> MRGLRKEALEELMKLLNMKDFPYRIEGIDISHLQGKYTVASLVVFEDGFPKKGDYRRYKIEQDHPDDYESIRTVVKRRYSKHPLPNLLFVD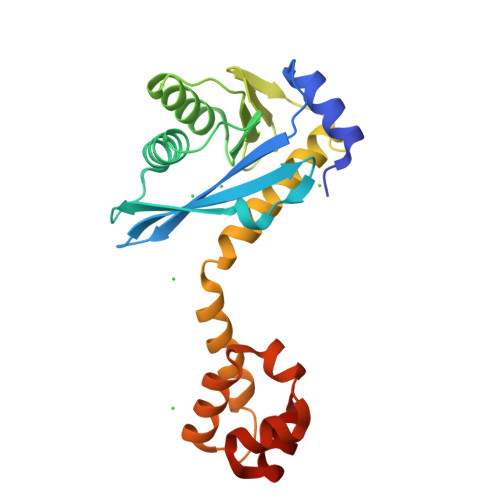GGIGQVNAAIEALKEIGKDCPVVGLAKKEETVVFENREIHLPHDHPVLRLLVQIRDETHRFAVSYHRKRREKESLRSVLDNVPGIGPIRKKKLIEHFGSLENIRSASLEEIARVIGSTEIARRVLDILG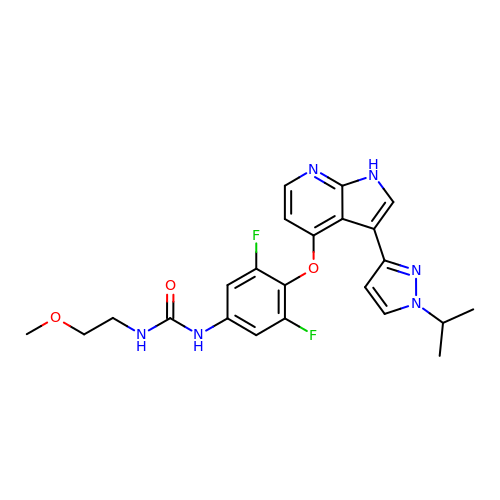1-[3,5-bis(fluoranyl)-4-[[3-(1-propan-2-ylpyrazol-3-yl)-1~{H}-pyrrolo[2,3-b]pyridin-4-yl]oxy]phenyl]-3-(2-methoxyethyl)urea | C23 H24 F2 N6 O3 | AMSRRTXLQMAOQA-UHFFFAOYSA-N>[2x]GSNTGIGQHILKNPLIINSIIDKAALRPTDVVLEVGPGTGNMTVKLLEKAKKVVACELDPRLVAELHKRVQGTPVASKLQVLVGDVLKTDLPFFDTCVANLPYQISSPFVFKLLLHRPFFRCAILMFQREF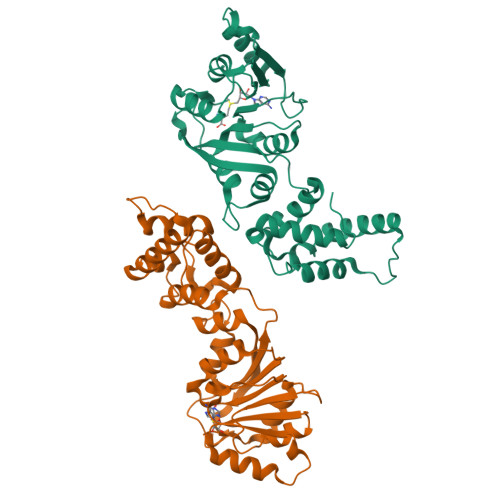ALRLVAKPGDKLYCRLSINTQLLARVDHLMKVGKNNFRPPPKVESSVVRIEPKNPPPPINFQEWDGLVRITFVRKNKTLSAAFKSSAVQQLLEKNYRIHCSVHNIIIPEDFSIADKIQQILTSTGFSDKRARSMDIDDFIRLLHGFNAEGIHFS>[6x]GPMSPLLHSLVGQHILSVQQFTKDQMSHLFNVAHTLRMMVQKERSLDILKGKVMASMFYEVSTRTSSSFAAAMARLGGAVLSFSEATSSVQKGESLADSVQTMSCYADVVVLRHPQPGAVELAAKHCRRPVINAGDGVGEHPTQALLDIFTIREELGTVNGMTITMVGDLKHGRTVHSLACLLTQYRVSLRYVAPPSLRMPPTVRAFVASRG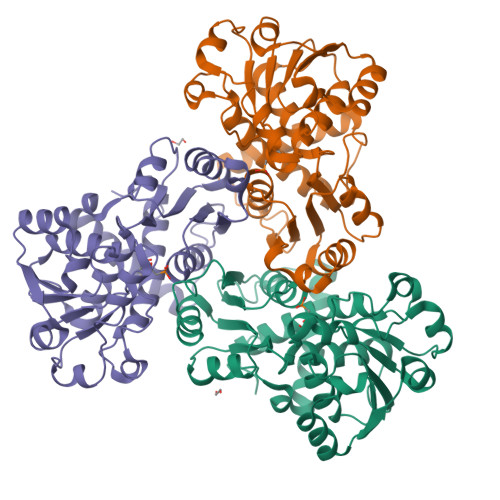TKQEEFESIEEALPDTDVLYMTRIQKERFGSTQEYEACFGQFILTPHIMTRAKKKMVVMHPMPRVNEISVEVDSDPRAAYFRQAENGMYIRMALLATVLGRF> MDHSITASYYDTTQQLSLLKHVLSEDKRPIAFIIAAGCPVSIRHNDAPLIPDVAGLTRKISDSFGGNPDSLLMKIIQNLKTTIPNPTIEDILSYIRLLQQIPMSGKIHDVENSVINALEESICELIEEEVNVDLPGNATPYHKIAAWINSINREHQVEIFTTNY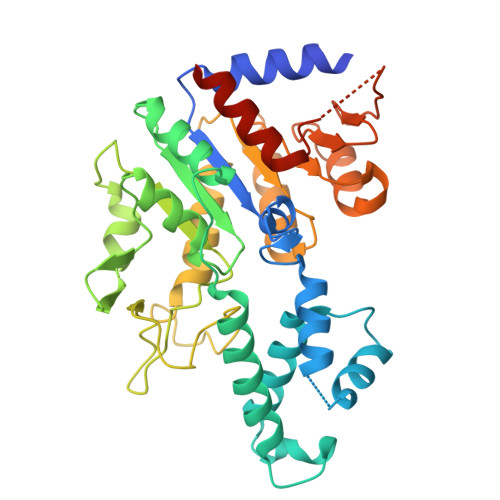DLLMEQALEELNVPYFDGFVGSKRAFFDIRTIEENKLPSRWSKLWKLHGSINWQLDKQTQTIWRGTPSKGCSLIHPSHLKYDQSRKMPYLVMMDQLKLFLNQPSAILITCGYSYKDQHINEVLSQGLQTNPNALIYGLQYDVLENYQEAKDMALKRSNLILLAKDRAIIGKKEGEWKPDPQSSQDNDPLLFFKLGDFQHLASFLEEISQYDWSKQND> SEISRVYEAYPEKKATLYFLVLGFLALIVGSLFGPFQALNYGNVDAYPLLMHHHHHHAVRASEISRVYEAYPEKKATLYFLVLGFLALIVGSLFGPFQALNYGNVDAYPLLKRLLPFVQSYYQGLTLHGVLNAIVFTQLFAQAIMVYLPARELNMRPNMGLMWLSWWMAFIGLVVAALPLLANEATVLYTFYPPLKGHWAFYLGASVFVLSTWVSIYIVLDLWRRWKAANPGKVTPLVTYMAVVFWLMWFLASLGLVLEAVLFLLPWSFGLVEGVDPLVARTLFWWTGHPIVYFWLLPAYAIIYTILPKQAGGRLVSDPMARLAFLLFLLLSTPVGFHHQFADPGIDPTWKMIHSVLTLFVAVPSLMTAFTVAASLEFAGRLRGGRGLFGWIRALPWDNPAFVAPVLGLLGFIPGGAGGIVNASFTLDYVVHNTAWVPGHFHLQVASLVTLTAMGSLYWLLPNLTGKPISDAQ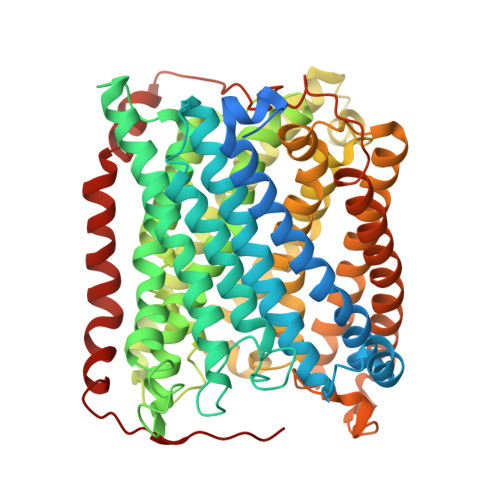RRLGLAVVWLWFLGMMIMAVGLHWAGLLNVPRRAYIAQVPDAYPHAAVPMVFNVLAGIVLLVALLLFIYGLFSVLLSRERKPELAEAPLPFAEVISGPEDRRLVLAMDRIGFWFAVAAILVVLAYGPTLVQLFGHLNPVPGWRLW>APQAPASATPAKVPVIEWGKCEQLKPSESERTSKAAVVDKCLQSLPLPDP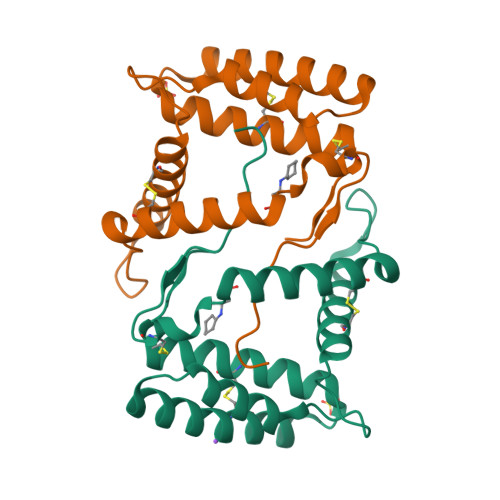EKATQQEIDKHRESVTTCALKAEGWFDDEGVYKFDRARNEIKNKKLDSEVEEAVLLKHDACQKEATEKHDDYINQVQLYQACMDYNISQICGIKVMV[2x]> MALVVQKYGGSSLESAERIRNVAERIVATKKAGNDVVVVCSAMGDTTDELLELAAAVNPVPPAREMDMLLTAGERISNALVAMAIESLGAEAQSFTGSQAGVLTTERHGNARIVDVTPGRVREALDEGKICIVAGFQGVNKETRDVTTLGRGGSDTTAVALAAALNADVCEIYSDVDGVYTADPRIVPNAQKLEKLSFEEMLELAAVGSKILVLRSVEYARAFNVPLRV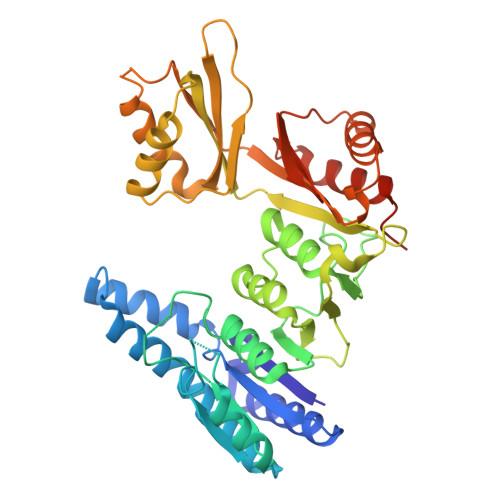RSSYSNDPGTLIAGSMEDIPVEEAVLTGVATDKSEAKVTVLGISDKPGEAAKVFRALADAEINIDMVLQNVSSVEDGTTDITFTCPRSDGRRAMEILKKLQVQGNWTNVLYDDQVGKVSLVGAGMKSHPGVTAEFMEALRDVNVNIELISTSEIRISVLIREDDLDAAARALHEQFQLGGEDEAVVYAGTGR> MKSGIYQIKNTLNNKVYVGSAKDFEKRWKRHFKDLEKGCHSSIKLQRSFNKHGNVFECSILEEIPYEKDLIIERANFWIKELNSKINGY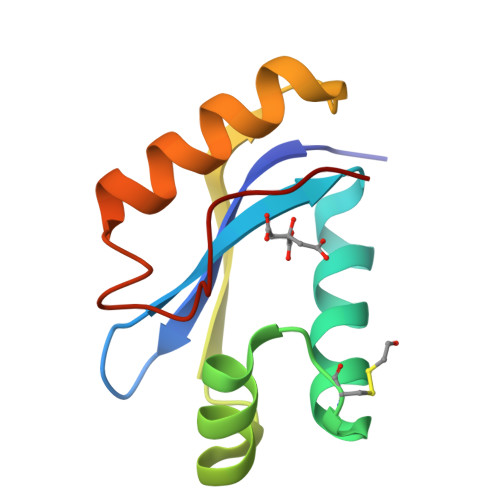NIADATFG> MGEYIKLKVIGQDSSEIHFKVKMTTHLKKLKESYCQRQGVPMNSLRFLFEGQRIADNHTPKELGMEEEDVIEVY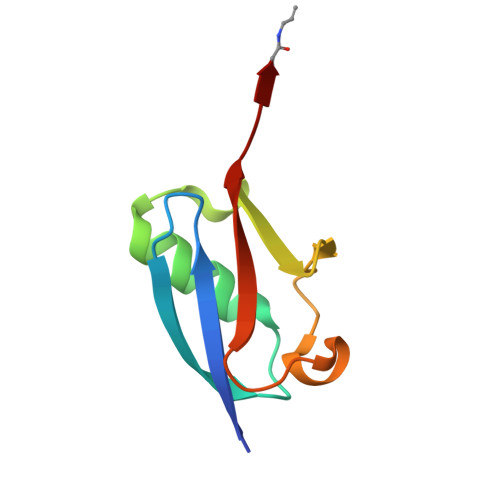QEQTGX>[6x]GPGHMMAAEAWRSRFRERVVEAAERWESVGESLATALTHLKSPMHAGDEEEAAAARTRIQLAMGELVDASRNLASAMSLMKVAEL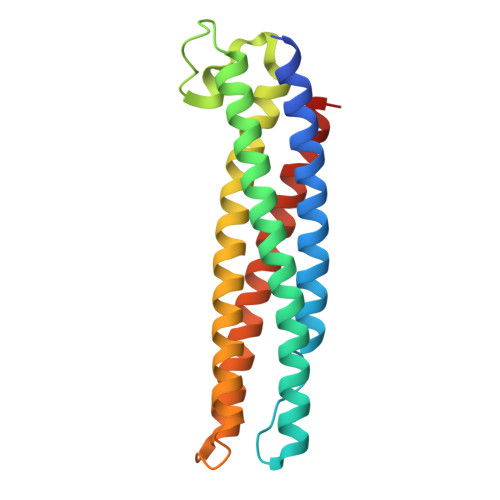LALHGGSVNPSTHLGEISLLGDQYLAERNAGIKLLEAGKDARKAYISVDGCRGNLDAILLLLDHPRVPCVDDFIEEELFVAGDNLQGAIGNAKLGTERAVGARQDVSGAN3-[5-[[(3~{R},4~{R})-3-ethyl-4-methyl-5-oxidanylidene-3,4-dihydropyrrol-2-yl]methyl]-2-[[5-[(~{Z})-(4-ethyl-3-methyl-5-oxidanylidene-pyrrol-2-ylidene)methyl]-3-(3-hydroxy-3-oxopropyl)-4-methyl-1~{H}-pyrrol-2-yl]methyl]-4-methyl-1~{H}-pyrrol-3-yl]propanoic 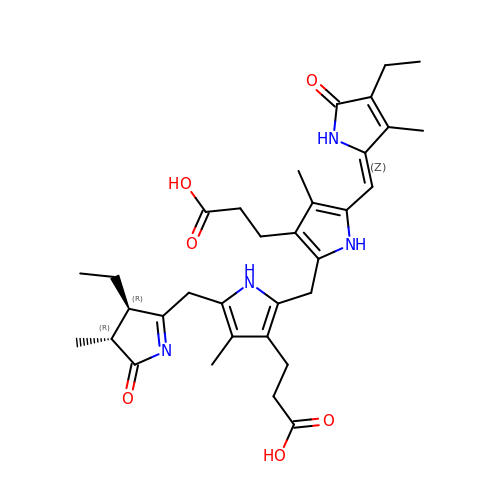acid | C33 H42 N4 O6 | RIXXCMVADHNPLY-UKJJQICTSA-N5-[2-[(2~{S},3~{R},4~{S},5~{R},6~{R})-6-(hydroxymethyl)-3,4,5-tris(oxidanyl)oxan-2-yl]oxyethylcarbamothioylamino]-2-(6-oxidanyl-3-oxidanylidene-4,9-dihydroxanthen-9-yl)benzoic 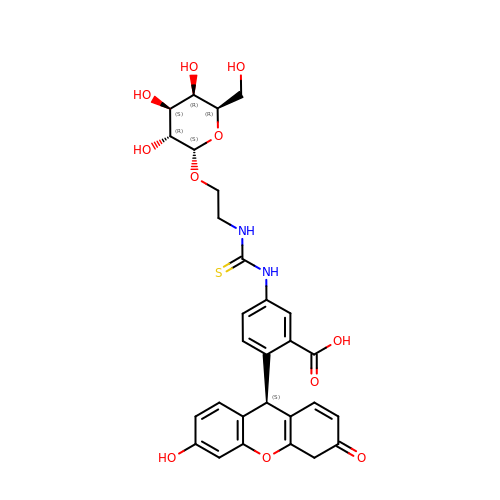acid | C29 H30 N2 O11 S | VPENXLROBWFVHN-RFDUDFTJSA-N> MDNKLDVFRRELVDVEGIPLFWSIAEHWSQVESFEARPDDILISTYPKSGTTWVSEILDLIYNNGDAEKCKRDAIYKRVPFMELIIPGITNGVEMLNNMPSPRIVKTHLPVQLLPSSFWKNDCKIIYVARNAKDVVVSYYYFYQMAKIHPEPGTWEEFLEKFMAGQVSFGPWYDHVKSWWEKRKEYRILYLFYEDMKENPKCEIQKI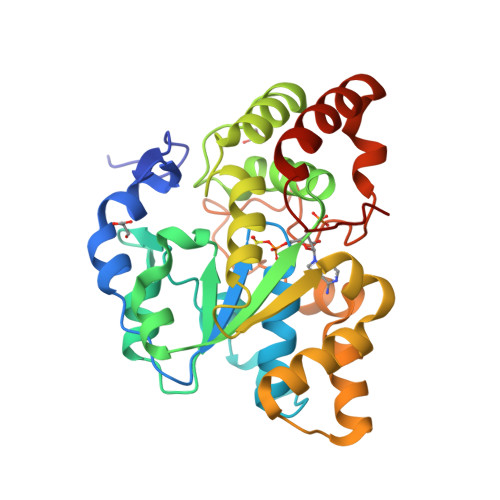LKFLEKDIPEEILNKILYHSSFSVMKENPSANYTTMMKEEMDHSVSPFMRKGISGDWKNQFTVAQYEKFEEDYVKKMEDSTLKFRSEI>[4x]MKKTKIVCTIGPKTESEEMLAKMLDAGMNVMRLNFSHGDYAEHGQRIQNLRNVMSKTGKTAAILLDTKGPEIRTMKLEGGNDVSLKAGQTFTFTTDKSVIGNSEMVAVTYEGFTTDLSVGNTVLVDDGLIGMEVTAIEGNKVICKVLNNGDLGENKGVNLPGVSIAL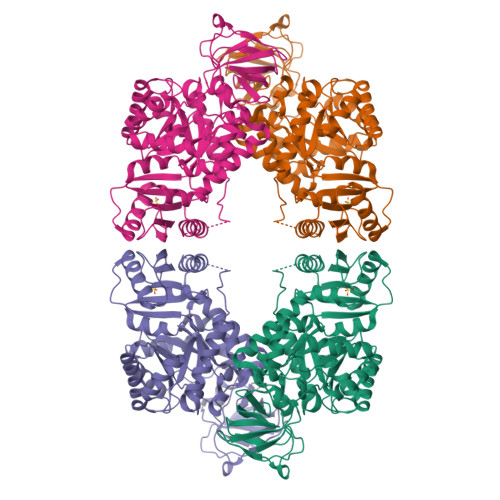PALAEKDKQDLIFGCEQGVDFVAASFIRKRSDVIEIREHLKAHGGENIHIISKIENQEGLNNFDEILEASDGIMVARGDLGVEIPVEEVIFAQKMMIEKCIRALKVVITATMMLDSMIKNPRPTRAEAGDVANAILDGTDAVMLSGESAKGKYPLEAVSIMATICERTDRVMNSRLEFNNDNRKLRITEAVCRGAVETAEKLDAPLIVVATQGGKSARAVRKYFPDATILALTTNEKTAHQLVLSKGVVPQLVKEITSTDDFYRLGKELALQSGLAHKGDVVVMVSGALVPSGTTNTASVHVL(2S)-3-carboxy-2-hydroxy-N,N,N-trimethylpropan-1-aminium 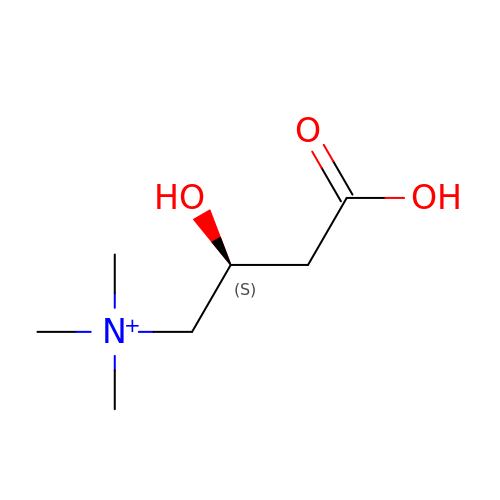| C7 H16 N O3 | PHIQHXFUZVPYII-LURJTMIESA-O>SNAKPTMLTPLEAGVE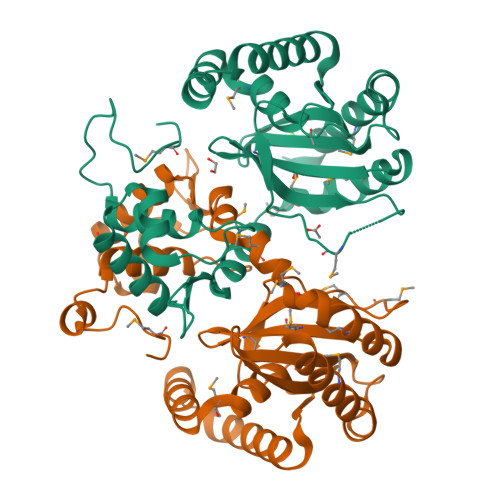EEDRQFVTALARGLEVLRCFTPTENTLGNQEIAHKTGLPKPTVSRLTHTLVRLGYLRQDALSGLYQLDIGILRLGYAMLSNLMIRTVASPLMQVLADYAKAAVAMAARDRLSMVYLDVVQGEGNMTMRRQIGSTLPLAGSSVGRACLAAMPEDERTFILEHIREREPENWPSIRKGLDRALRDFEDYGYCLSIGEWHRDVNSVAVPLVHKQYGVLVFNCGGPSFQLPREKLEDDIGPRLIEMVHNISSAVP[4x]> MNRFFTLLFFVLFFNAAINFVSSHRIVGYYQGIRPLTNDQAKKLTHLILAFSTPDSQGNLSPLSSVLKQALKAGKSANGALKVMIAIGGGGFDPAIFTSLAS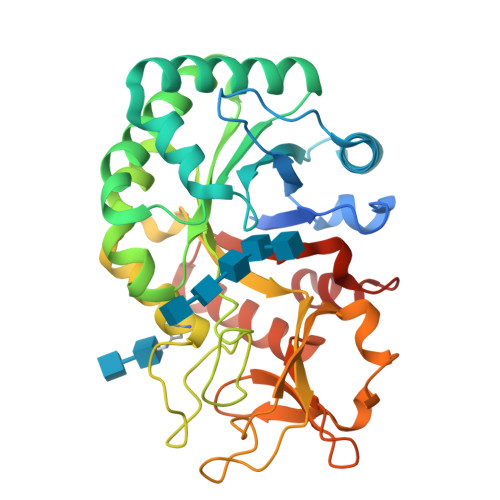NSGTRKSFINNIVSYLKTNELDGCDIAWAFPTSSDKAIFVTFLRDLKKAMAPSGAVLSMASAASAFYLDPGYDLPGIESAVDFINVMCYDYYGSWTKTSTGPNSPLFKGGSADPSDTLNSNWTMNYHLMKVYNRAKLNMGVPFYGKSWTNVGAPLNGDGLWRQLGTYGTELAWRNMGKSFDMTKTTYHKTAKTAYIYDTATKNFLTFDNPQSLKDKAKYVAEKGIGGIMIWSIDQDDDKLSLLNSVSYHHHHHH> MHHHHHHKNIINTSILNLRYESNHLIDLSRYASKINIGSKVNFDPIDKNQIQLFNLESSKIEVILKNAIVYNSMYENFSTSFWIRIPKYFNSISLNNEYTIINCMENNSGWKVSLNYGEIIWTLQDTQEIKQRVVFKYSQMINISDYINRWIFVTITNNRLNNSKIYINGRLIDQKPISNLGNIHASNNIMFKLDGCRDTHRYIWIKYFNLFDKELNEKEIKDLYDNQSNSGILKDFWGDYLQYDKPYYMLNLYDPNKYVDVNNVGIRGYMYLKGPRGSVMTTNIYLNSSLYRGTKFIIKKYASGNKDNIVRNNDRVYINVVVKNKEYRLATNASQAGVEKILSALEIPDVGNLSQVVVMKSKNDQGITNKCKMNLQDNNGNDIGFIGFHQFNNIAKLVASNWYNRQIERSSRTLGCSWEFIPVDDGWGERPL

Botulinum neurotoxin (BoNT) is the active agent that causes the deadly condition botulism. The smaller 50 kDa light chain (LC) possesses a single zinc-endopeptidase domain whereas the larger 100 kDa heavy chain is comprised of two domains—a target cell receptor binding (HC) domain and a translocation (HN) domain. The BoNT HC domain is responsible for targeting the toxin to a specific cell type and the specific receptors involved have been identified for most serotypes. As with all reported structures of the BoNT receptor binding domain, present is a characteristic β-jellyroll fold at the N-terminal half and a predominantly β-trefoil fold at the C-terminal half of the protein.

We have identified a single crystallisation condition that produced two crystal forms of HC/A1—one possessed the equivalent disulphide bond whereas the other did not. Using 25% w/v PEG 1500 and 0.1 M MIB pH 4.0, HC/A1 crystallised into orthorhombic crystals with the space group P212121 (crystal form 1) that diffracted to a resolution of 1.45 Å. No disulphide bond was observed in this structure. Instead, Cys1235 rotated away from the junction due to a backbone rotation, bringing the neighbouring Lys1236 toward Cys1280. Our findings suggest that the crystallisation condition is not the only determinant as to whether the bond is present or not. For example, serotype /A binds to a glycosylated luminal domain of the synaptic vesicle 2 (SV2) protein, preferentially to the C isoform (SV2C), as well as a ganglioside, namely GT1b.(2S,3R,4R,5S,6S)-2,3,4,5,6-PENTAHYDROXYCYCLOHEXANONE 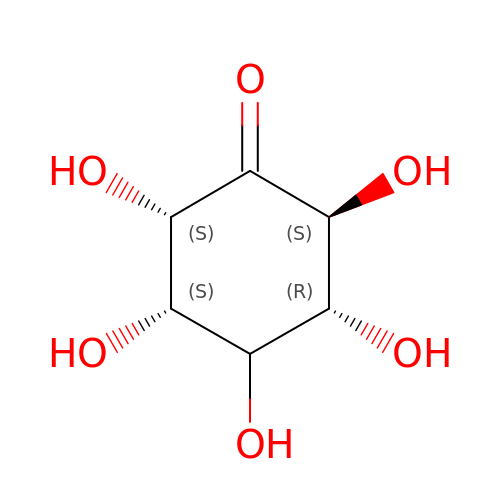| C6 H10 O6 | VYEGBDHSGHXOGT-REJXVDBHSA-N>[2x]MGSSHHHHHHSSGMVFYFTSSSVNSSAYTIYMGKDKYENEDLIKHGWPEDIWFHVDKLSSAHVYLRLHKGENIEDIPKEVLMDCAHLVKA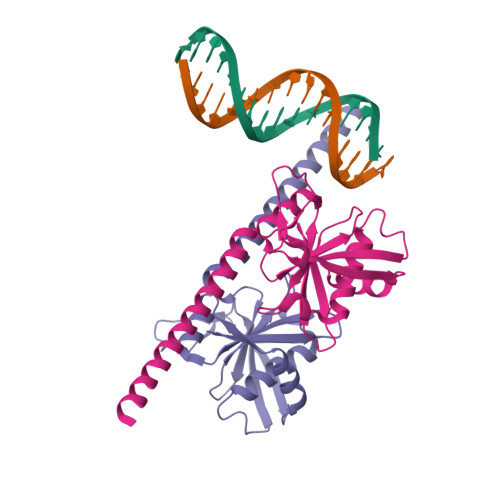NSIQGCKMNNVNVVYTPWSNLKKTADMDVGQIGFHRQKDVKIVTVEKKVNEILNRLEKTKVERFPDLAAEKECRDREERNEKKAQIQEMKKREKEEMKKKREMDELRSYSSLMK>EEGQKVDHCARHGEKLLLFCQEDSKVICWLCERSQEHRGHHTFLMEEVAQEYHVKLQTALEMLRQKQQEAETERNQVAKRVPKAPPEEK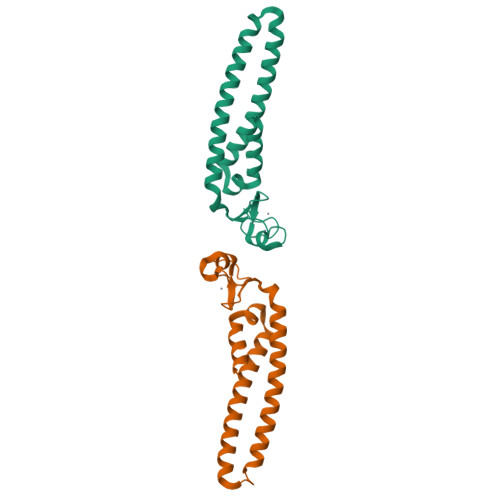EALIARGKALGEQTQYMRELISELEHRLQGSMMDLLQGVDGIIKRIENMTLK[2x]>MANPTLFVSYDQNGKKLSFANWISVLSPQDTPFVSMTGKESINQTIFSWQTDALASVDGNNAHVEGSRAEDGEMKPTVIKSNVTQILRKVVRVSDTANTTANYGRGRELMYQLEKKGKEIKRDLEKILLSGQARTDVLADQYLTNSAADPAVAGLNDTHAARKTGAFQFLCAHGGLAGGVVDKTKNGPADPDTGAVTVKVAQNASNPTTNIGFDEADIFDMTLQLYTAGSEADIIMINPAHAKIFAGLQENTQGSRKRIFENTKQFIYEVNSITDPLGQSYKIIVNRWMPTDAVYFFRSADWTQMVLRAPKRTELAKDGSYEKWMIEMEVGLRHRNPYASGVLFTAAGKAAA[95x];>MAIETNAVVITDLNPLYPRDRDYIYEGAAQIRLIKQTLQNTFPNVTEPVDIDSDTFKIMSEKLKFTGDAMDVGGLMIKNVTPGTGDKDVVTKGQMEAFMKNWMENKLYRIGSYYITEEDINPGDSISLGFGSWAKVTGVIMGTGVVNPDGSVPNAQRVEFQAGGTGGRVFNTIRTENVPLMTVNGSSFSLSSNTHSHNMVFGRGDASGHNSSPNWYSPGGGYSQRTDNDTHTHTISGSVSLGRDDISRQPINTLPPFRAAHIWRRIS[3x];>[2x]MAMPDVQYPINTYGWLKKAVALWADRDDDEFVNQIPNFINFAEKEIYRNLRIPPLEKEVYLDIKDGVAYIPPDYLEAQWMMRAKDGTIFQVTSPEEISYRRQHGTINPSHWNNQPVNFARFGSRFIFYPSIEADTPYYPDDGSPLIPAENSVILSYYADPPEFHEDTDTSTILTIAPELLLYFTLRHACLFVQDDNGVQKWSALGKAILDEMVEQNKKQEYSGSPIAIPNNMTRLQSSLPDIYGIRTSRV;> MALYPIKSLGAVGVIADQAPTDLAPNAFTNAINARFVEQRVFKTGGNAPLSYVDEDKDLTPLSFVSMPFDYYSAGNSFLVVGTNKKLYKLTDESLTDISRKVATVTKKASASIKIYPVVSQIVPKESTISMNFNQTKNLEVSLLPADANNTNLIWEVSNSSYGSITVDPSDSKLATLTSFEKEGNLVVTISTANESVVAQIAVNIIDGDSGIFLSQDTVTIRKGGTTTLTAVTGKTPVTWSSNNASIVSVTPNANSLTAVITANGEGNVTITADNGTKTASCEIVSIPQIDSISLSQSDVTVSRGSQYILTATLSPANAPNQNITWTSSNPNIATVSGTSTQGTINALLAGFTEITATTEEGNRVAVCTVRVDLAGRTMRTSAMAFAAPVSESVETQEEEVVTPPESEETVYFAEPTSGIDTSGMYEGNNFYDYSNVNDIEGFARASLLATPLSSVTLDIVSASLDVGEEIVITATASPEGEYSYQWSVDKTGYVSTTSVTGKSIKLVALRKGEINVTCTVSQMTQKDYDAFDDYPWYHAVISNCAVATTHYETPQVKEFESEYFVDLPGWGEQTVVDNDGNPSVKKFNWKCERVRSFNNRLFALNMREANASGVTTNYPLRLRWSNFANENKAPTLWDDFAYDRVVSSDLASNIVGQTQALENGYAGYIDLADSNGSLIDILPLKDYLFVYTEFETYIGSPTNNTYQPLMFKKLFNDSGILAPECVVEVEGSHFVVTQNDVILHNGATKKSIASNRVKNMLINEVCLVNPLATRVHLHQDKKEVWVLYVGPGEPKESFACTKAAVWNYEFDTWSFRTIPYAQCIGLVDPPVLERGPIWSDFQEITWDDPSIKELVWRKDATNFRQRVTIVGSFLKGFYQVDVGALDYFYDRLNDVVIEKPLEMRLERTGIDFDNVTNEWNQKHINRFRPQTTGSGTYIFEAGGSQFSNEYGHPHTSKTYTIGVDRHVSVRLNHPYLFYNVIDNDVNSNAAINGLTIEFAVGGRR;>[3x]MIVYNNQAPDAVNNVGQFGATEGSIGAYKQAAEYAADSKYWALLAESKFGTIDDLIAEVERLYQQGVLMKQDIEDLKQDFKDQDARLMSLIAQTNAAVSDANNAVALINQKLIEVQNQLDVLLGMSVDVTTLPPGTPATGSFNPNTGVISLGIPEGEPGKDGSVKDLDTAPTGVPELGDLGFYVDKDDNTVHKTTLENIANLTPSVRSVSVNGGPALDGEVALTINKETVGLGNVLNVAQYSRQEINDKFDKTTKTYQSKAEAYADAQYRQVGEKVLVWEATKYEFYTVAANKTLTPVKTEGRILTVNSRSPDSSGNIDITIPTGNPSLYLGEMVMFPYDPSKNISYPGVLPADGRLVSKESASDLGPSLVSGQLPVVSETEWQSGAKQYFSWGKLADGITDADSTNFINIRLPDWTGGEAIRAPDSDKDSQYNGSVQAQKPYVVTVNNQAPDEITGNVNISRSILGAASSGANSDITSLSGLTTPLSISQGGTGAKDAASARSNLGLGSVSTLDNVPIASGGTGAGDAAGARFNLGLGNSATMNTGTNSDNVLKVGDFGIGRPDGALVFDTTSQDQLLAGLDTYGLCVFRNNQQIAAPWDIWNYSSNLFFRAGDTYSMISIPFESAGKIKVFGGASGSGWKTSRTVYDTVNTTVDVNGFIKAASPIVKVFHDGSFETNEQSDGVSVKKISTGVYLISGCLGLNSDAGWGGVDGGFEIPIDRNKQPRVWLDYEVKEDGSLLIKTYHRTHSTSPAFARNELEGFSDGDPVDIPKDAFISVRVEMPSK;>MGAGGFRKNTGRNNTTLPYNVGFLNNVQDTETYNVAVYDELQKVSTATNQMFQAIDEIHEEIDVRIKALNAMNLQFDELENRITTEIETAIADIQTQMGNLSTEDIWDNSVQPPVKLESTVSGFKTSIEGNTTKIQTVEGIVNDQGQEIALVQTELQNINGSLSQYMKLSEYEATWGVNSTVNGRYAGVKLTNNGTNSQFQVTANKFIVGDGSSGNTPFVFEGGRARMEFADIKNVNITTAQIANARIQWAQIDNVSISNAQIQNLSADKITAGSMWGSNWRLTVGGDFVMGGTGGAQLWMNGNRIDFYDGSGALRIRIGSW[3x];>[2x]MAKQKYSEEVLDELRVDLQRRFNYAQGYVDMAVKGYAREAWEYFYGNLPAPVTAGSSSWVDRTVWESVNGTLQDIINVFCSGDEAVTFVADNQQDSDAADVATKLVNQILLRDNPGYNIISSAAQECLVTRNSFIKYYWDEQTSTQTEEAEGVPPEALAAYVQGLEAGGLKNLEVFTEENEDGTVDVKVTYEQTVKRVKVEYVPSEQIFVDEHATSFADAQYFCHRVRRSKEDLVAMGFPKDEIEAFNDWTDTMDTTQSTVAWSRTDWRQDIDADIGTDTEDIASMVWVYEHYIRTGVLDKNKESKLYQVIQAGEHILHTEEVTHIPFVTFCPYPIPGSFYGQSVYDITKDIQDLRTALVRGYIDNVNNANYGRYKALVGAYDRRSLLDNRPGGVVEMERQDAIDLFPYHNLPQGIDGLLGMSEELKETRTGVTKLGMGINPDVFKNDNAYATVGLMMNAAQNRLRMVCRNIAHNGMVELMRGIYNLIRENGEVPIEVQTPRGMIQVNPKQLPARHNLQVVVAISPNEKAERAQKLISLKQLIAADAQLAPLFGLEQDRYMTAQIFELMGIKDTHKYLLPLEQYQPPEPSPMEILQLEMTKAQVENVQASSQKMIADAFDQRERTTFEQQKAADELSLRQEELQFKQENAADAMTLENRKEDNNATLEQAKHKLALMQQQVRQYESVLKELQMVMSHQVDQEKIVQQARVQDKTLELQKKEANVTKKEQQASLKDSRIPGKRLGSKK

Escherichia coli phage SU10 belongs to the genus Kuravirus from the class Caudoviricetes of phages with short non-contractile tails. Here we show that the virion of SU10 has a prolate head, containing genome and ejection proteins, and a tail, which is formed of portal, adaptor, nozzle, and tail needle proteins and decorated with long and short fibers. In contrast to other short-tailed phages, the tails of Kuraviruses elongate upon cell attachment. After binding to the host, SU10 tail, nozzle proteins, and short fibers re-arrange to form a nozzle that extends the tail.

The virion of bacteriophage SU10 has a prolate head with a length of 1430 Å and a diameter of 460 Å, which is formed by the major capsid protein (gp9). The tail is 220 Å long and decorated with six long and six short tail fibers. The tail is attached to one of the vertices of the prolate capsid, where the dodecamer of portal proteins (gp6) replaces a pentamer of capsid proteins. The part of the portal complex protruding from the capsid enables the binding of the dodecamer of adaptor proteins (gp11). A hexamer of nozzle proteins (gp17) is attached to the adaptor complex and enables the binding of six short tail fibers, trimers of short tail fiber protein (gp16). The tail needle, which is formed by three polypeptide chains (gp18), protrudes from the central channel formed by the nozzle proteins. In the SU10 virion, the short tail fibers are tilted towards the capsid and the tail needle protrudes from the tail complex. The 260-Å-long tail needle protrudes 200 Å from the nozzle complex. The cryo-EM density of the genome in the SU10 virion was resolved in both fivefold symmetric and asymmetric reconstructions of its head.> 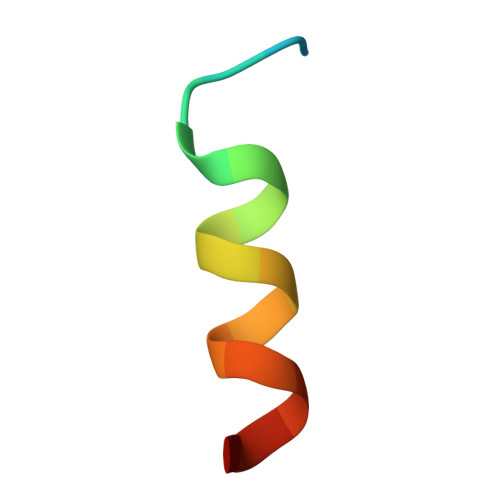XDPAHWYCDFAAQVCNFSX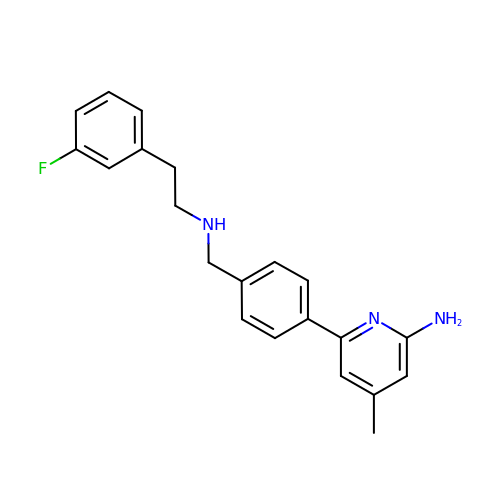6-[4-({[2-(3-fluorophenyl)ethyl]amino}methyl)phenyl]-4-methylpyridin-2-amine | C21 H22 F N3 | YIRCIVHQWVHKOD-UHFFFAOYSA-N Phycoviolobilin, blue light-absorbing 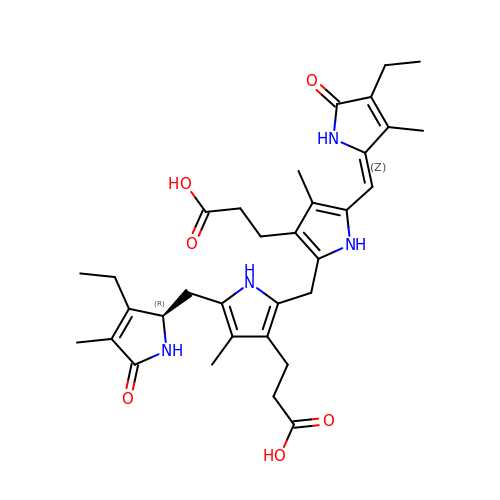form | C33 H42 N4 O6 | KTSIPBCNIBDFRK-JTNIOKRPSA-N> SGIIG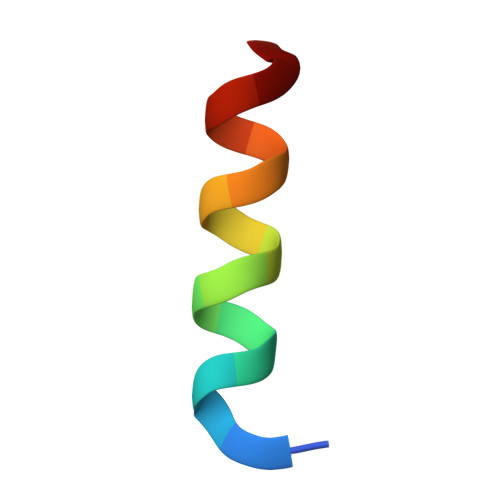NLRHMALDMGNE> RPHPDHELVVCGAPDAAALTGLLTRVRAAATALSRPELTDLAAGLAAAHRGDVPARFAAAVRDADGLVAALDRALGHLAEGGRRLLDAGRGLFLVVGGPLRVGLLFPGQAAPVHADRGALGHLLGDADAGTGSDPDSGVKPAEPVDTAVAQPAIIADSLAGIRWLDRLGARPVGALGHSLGELAALSWAGALDADDTLALARARGEAMSAATEAPSGMLSLRADLAAARELAAGTGAVVAVDNGERHVVVAGTRPELDRVAEAARHAGIEATPLAVSHAFH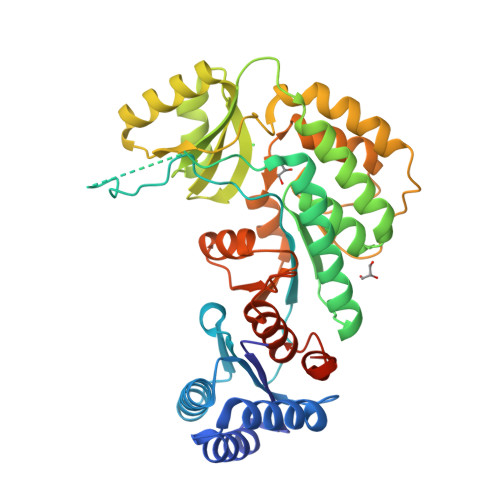SPLMAPAAEALRRAAGRLPWRRPERPVASTVTGAWWADEDPVEVLVRQLTGPVRFREALGLLDADLLVEVGPGRMLSALAEAAGRTAVSLDAGAASAAGMAAGTAALFAAGAVDDATPFFAGRFTRPFDRDREREFLVNP> NTKYNKEFLLYLAGFVDSDGSIIAQIKPNQSVKFKHRLQL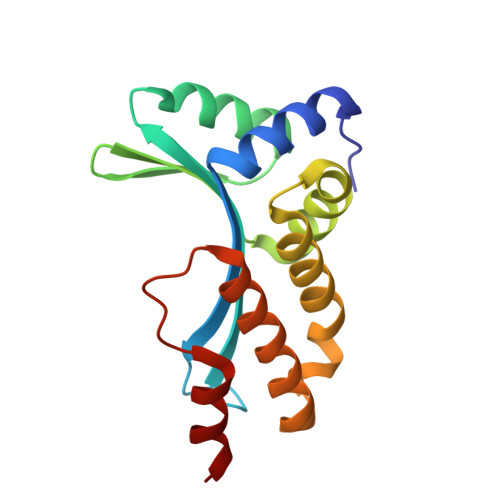TFDVTQKTQRRWFLDKLVDEIGVGYVADSGSVSKYRLSEIKPLHNFLTQLQPFLKLKQKQANLVLKIIEQLPSAKESPDKFLEVCTWVDQIAALNDSKTRKTTSETVRAVLDS> MGSSHHHHHHENLYFQGMMFKKKMLAATLSVGLIAPLASPIQESRANTNIENIGDGAEVIKRTEDVSSKKWGVTQNVQFDFVKDKKYNKDALIVKMQGFINSRTSFSDVKGSGYELTKRMIWPFQYNIGLTTKDPNVSLINYLPKNKIETTDVGQTLGYNIGGNFQSAPSIGGNGSFNYSKTISYTQKSYVSEVDKQNSKSVKWGVKANEFVTPDGKKSAHDRYLFVQSPNGPTGSAREYFAPDNQLPPLVQSGFNPSFITTLSHEKGSSDTSEFEISYGRNLDITYATLFPRTGIYAERKHNAFVNRNFVVRYEVNWKTHEIKVKGHN

Leukotoxin ED (LukED) is one of these bicomponent pore-forming toxins that Staphylococcus aureus produces in order to suppress the ability of the host to contain the infection. The bicomponent pore-forming toxins have two separate water-soluble subunits, one of class S (related to the slow-eluted component of PVL) and one of class F (related to the fast-eluted component of PVL). The S subunit is typically involved in targeting the specific cell type via the interaction with surface receptors and in the recruitment of the other toxin subunits, leading to oligomerization and the formation of an octameric prepore. The prepore is composed of alternating S and F subunits and is able to assemble a β-barrel pore domain in the cell membrane, producing the mature pore that ultimately induces cell death by osmotic lysis.

Crystals of LukE12–311 and LukD27–327 provided measureable X-ray diffraction data to 3.2 and 1.7 Å resolution, respectively. Each of the two crystal structures had one molecule in the asymmetric unit, and the two refined models included amino acids 30–311 of a total of 311 for LukE and amino acids 27–325 of a total of 327 for LukD. LukE–HlgA superimposition results in an r.ms.d. of 0.53 Å. Indeed, LukE targets CCR5 to kill inflammatory macrophages, dendritic cells and T cells. Furthermore, LukE binds CXCR1 and CXCR2 and previous studies have identified the L3 loop in the rim domain as the binding region. The crystal structure of LukE provides insight into the residues required for receptor identification. We argue that the structural features that determine the binding of LukE to CXCR1/CXCR2 receptors in contrast to LukS-PV are dependent on the presence of glycine and proline residues in loop L3 (Pro212, Gly214, Pro215 and Gly217) as well as a different distribution of polar residues (Gln210, Asn213, Thr216 and Ser211). The fact that loop L3 in LukE is one residue longer compared with the same loop in LukS-PV results in positioning residues Pro215-Thr216 so that the local solvent exposure is higher. Indeed, the solvent-exposed surface of loop L3 is 1750.8 Å2 in LukE and 1472.4 Å2 in LukS-PV with a different charge distribution. These important variations could explain the different specificity of binding of LukE and LukS-PV to chemokine receptors.> GPGYQDPGNIQIQSMPKVKERVSVPSKDDTIYSYHDSIKDSIKAVVNISTEKKIKNNFIGGGVFNDPFFQQFFGDLGGMIPKERMERALGSGVIISKDGYIVTNNHVIDGADKIK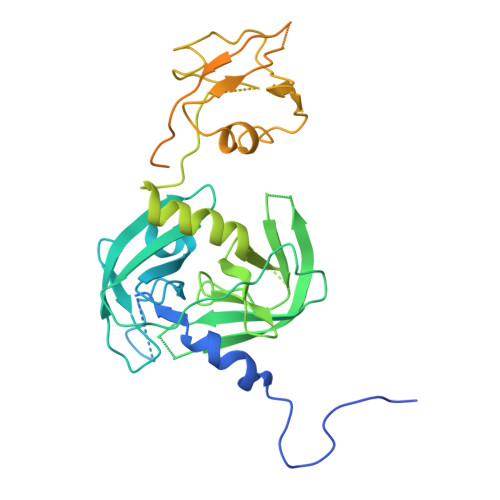VTIPGSNKEYSATLVGTDSESDLAVIRITKDNLPTIKFSDSNDISVGDLVFAIGNPFGVGESVTQGIVSALNKSGIGINSYENFIQTDASINPGNSGGALIDSRGGLVGINTAIISKTGGNHGIGFAIPSNMVKDTVTQLIKTGKIERGYLGVGLQDLSGDLQNSYDNKEGAVVISVEKDSPAKKAGILVWDLITEVNGKKVKNTNELRNLIGSMLPNQRVTLKVIRDKKERAFTLTLAERKNPNKKETISAQNGAQGQLNGLQVEDLTQETKRSMRLSDDVQGVLVSQVNENSPAEQAGFRQGNIITKIEEVEVKSVADFNHALEKYKGKPKRFLVLDLNQGYRIILVK> ETLVRPKPLLLKLLKSVGAQKDTYTMKEVLFYLGQYIMTKRLYDEKQQHIVYCSNDLLGDLFGVPSFSVKEHRKIYTM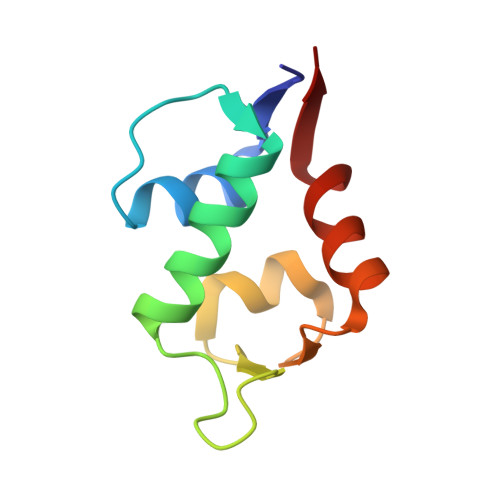IYRNLVVV> MSNLLTVHQNLPALPVDATSDEVRKNLMDMFRDRQAFSEHTWKMLLSVCRSWAAWCKLNNRKWFPAEPEDVEDYLLYLQARG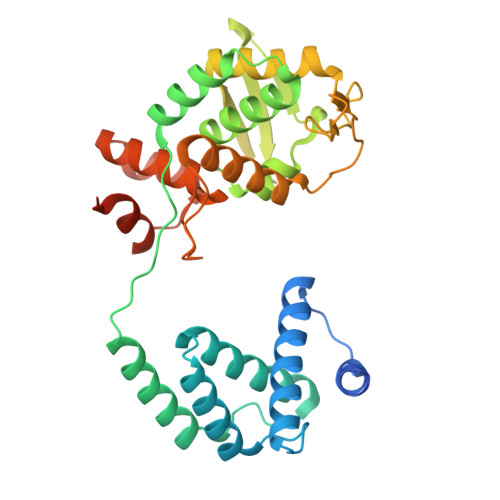LAVKTIQQHLGQLNMLHRRSGLPRPSDSNAVSDVMRDIRKENVDAGERAKQALAFERTDFDQVRSLMENSDRCQDIRNLAFLGIAYNTLLRIAEIARIRVKDISRTDGGRMLIHIGRTKTLVSTAGVEKALSLGVTKLVERWISVSGVADDPNNYLFCRVRKNGVAAPSATSQLSTRALEGIFEATHRLIYGAKDDSGQRYLAWSGHSARVGAARDMARAGVSIPEIMQAGGWTNVNIVMNYIRNLDSETGAMVRLLEDGD> NLFVALYDFVASG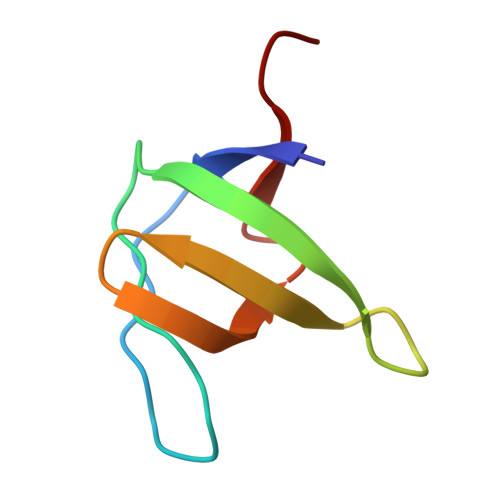DNTLSITKGEKLRVLGYNHNGEWCEAQTKNGQGWVPSAYITPVNS> GSGAWKASVDPLG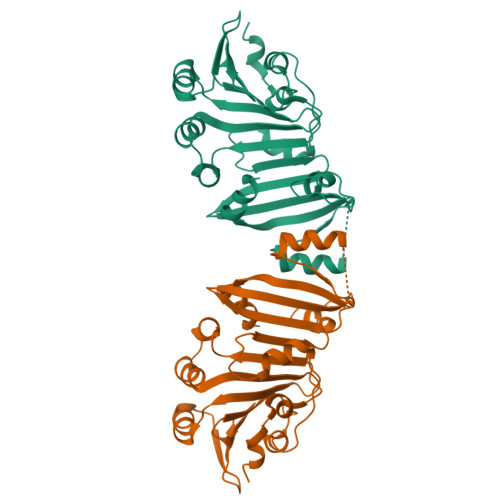VVGSGADVYLYFPVAGNENLISRIIENHESKADIKKIVDRTTAVYGAFFARSKEFRLFGSGSYPYAFTNLIFSRSDGWASTKTEHGITYYESEHTDVSIPAPHFSCVIFGSSKRERMSKMLSRLVNPDRPQLPPRFEKECTSEGTSQTVALYIKNGGHFITKLLNFPQLNLPLGAMELYLTARRNEYLYTLSLQLGNAKINFPIQFLISRVLNAHIHVEGDRLIIEDGTISAERLASVISSLYSKKGSS>[10x]MSEGRIPLIGEKFPEMEVITTHGKIKLPDDYKGRWFVLFSHPGDFTPVCTTEFYSFSKKYEEFKKLNTELIGLSVDSNISHIEWVMWIEKNLKVEVPFPIIADPMGNVAKRLGMIHAESSTATVRAVFIIDDKGTVRLILYYPMEIGRNIDEILRAIRALQLVDKAGVVTPANWPNNELIGDKVINPAPRTIKDAKMRLGQPFDWWFTYKEVKTT

Prx proteins reduce hydrogen peroxide and organic peroxides to water and the corresponding alcohols, respectively, by making use of a thiol-dependent mechanism involving catalytic cysteine residues. Archaeal Prxs belong to one of two subfamilies, BCP/PrxQ or Prx6, with the latter subfamily typically being 1-Cys Prxs that are characterized by a peroxidatic cysteine residue (CP), which is the sole redox-active cysteine, and thus lacking the resolving cysteine (CR) that is present in 2-Cys Prxs and forms a disulfide bond to the oxidized CP. Besides peroxidase activity, archaeal 1-Cys Prxs are moonlighting enzymes that also have a chaperone activity, thereby protecting proteins and DNA from damage caused by oxidative and thermal stress.

In contrast, no structural information was available about this Prx enzyme in Sulfolobus spp. Here, we describe the crystallization and structure determination of 1-Cys SiPrx from S. islandicus, a highly conserved homolog (95% sequence identity) of Bcp2 from the closely related S. solfataricus. For TkPrx, it has been shown that two C-terminal cysteines are responsible for a redox-dependent switch between a dimeric and a higher oligomeric state, with the former mainly functioning as a peroxidase and the latter mainly performing a molecular chaperone function. Intriguingly, while these C-terminal cysteines are highly conserved in all other archaeal 1-Cys Prxs, the Sulfolobus Prx6-subfamily 1-Cys Prx proteins lack both of them and only have a single cysteine that is the CP, thus evoking questions about its oligomeric state. The quaternary structure of 1-Cys SiPrx is similar to those of PhPrx and ApPrx. In this structure, 21% of the total accessible surface area of a monomer is buried upon dimerization. In contrast to the ApPrx structure, in which citrate was present in the active site, the H2O2-binding pocket of 1-Cys SiPrx was found to be empty. Taking into account the monomeric molecular weight of 24.7 kDa, we conclude that 1-Cys SiPrx mainly exists in a decameric oligomeric form corresponding to the quaternary structure observed in the crystal structure, and that a smaller population exists of a higher-order oligomer, which is probably a 20-subunit protein. Archaeal 1-Cys Prxs are characterized by a CXDWWFC motif in the C-terminal arm domain. Both cysteines are highly conserved in the archaeal enzymes and contribute to the redox-dependent association of dimers into higher-order oligomers.> PSDLACRLLGQSMDESGLPQLTSYDCEVNAP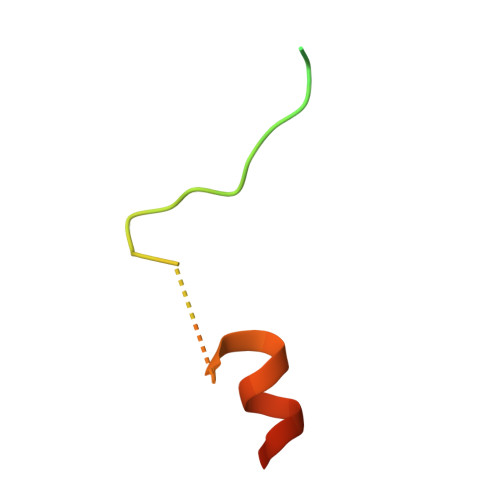IQGSRNLLQGEELLRALDQVN>[2x]AMATRQEEMIDHRLTDREWAEEW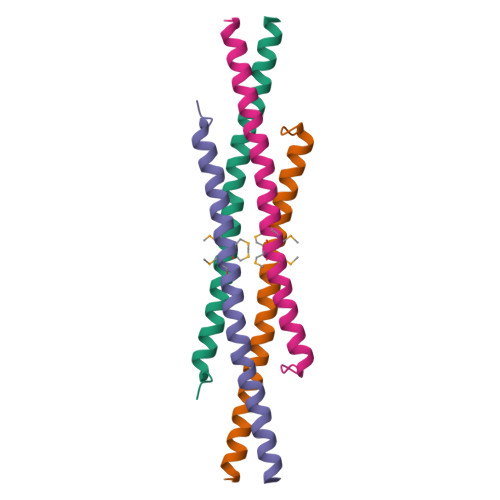KHLDHLLNCIMDMVEKTRRSLTVLRRCQEADREELNYWIRRYSDAEDLK> MKNIYNFLIYFIFCGIGAGCSSSSGEDFPAPESEPVDNSLIKKELCTEGASVEAKKVYTYLRNCWGRKTLSSTMANVTWNVNEAIWVNRQTGKYPAIACFDYMNLPASPADWIDYNKISVVEDWWNAGGLVAACWHWNVPVTENSSEYKCMISETDFDITKALQEGTRENEIIKADLEELAGYLLLLKQKNIPVIWRPLHEAAGKWFWWGKDAASYKRLWKLVYETFKQKGLNNLIWVWTSETNDRDWYPGDAYVDIIGRDVYHKTSAAGLATDFDALKKAFPDKLIALSE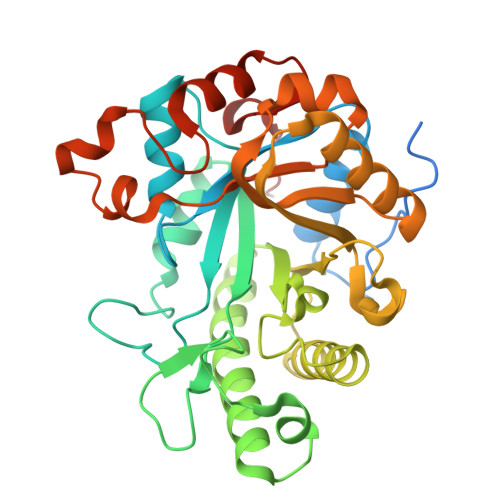CGDVATIDKQLAAGAQWAWFMTWYDYEVTKDTTAPVFNSGQHEHADKAWWNNAFGQPGVICRSDLPSFKLEHHHHHH> GGSPNGQTKPLPALKLALEYIVPCMNKHGICVVDDFLGKETGQQIGDEVRALHDTGKFTDGQLVSQKSDSSKDIRGDKITWIEGKEPGCETIGLLMSSMDDLIRHCNGKLGSYKINGRTKA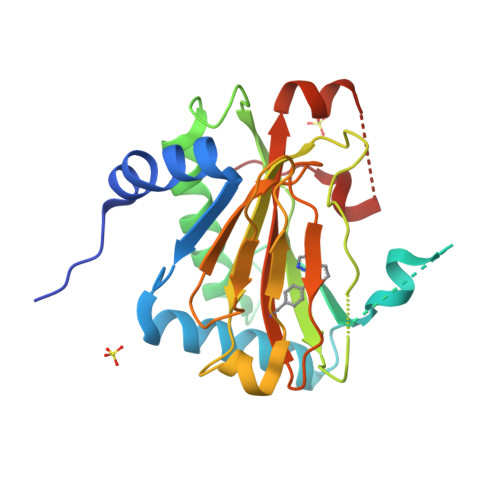MVACYPGNGTGYVRHVDNPNGDGRCVTCIYYLNKDWDAKVSGGILRIFPEGKAQFADIEPKFDRLLFFWSDRRNPHEVQPAYATRYAITVWYFDADERARAKVKYLTGEKGVRVELNK> MSEVKELLEEFLKRNKPVRIHHKNGEEIKVRITHIGEDTVEFELNGRTHRIN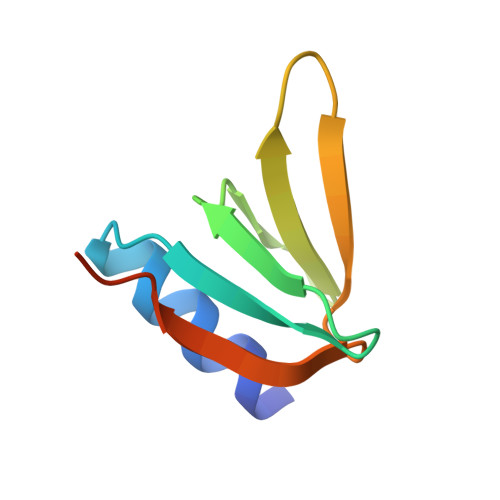IKDILDVKEWLEHHHHHH>[4x]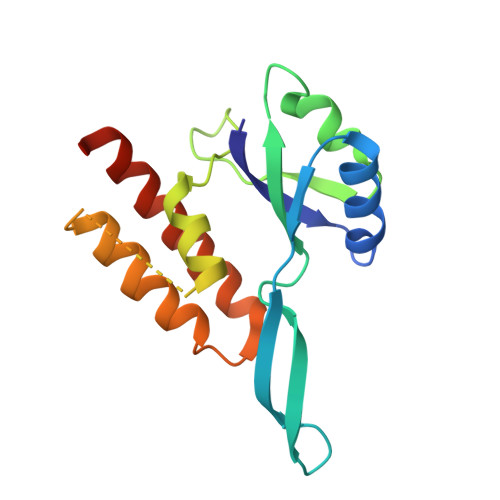MQSWYLLYCKRGQLQRAQEHLERQAVNCLAPMITLEKIVRGKRTAVSEPLFPNYLFVEFDPEVIHTTTINATRGVSHFVRFGASPAIVPSAVIHQLSVYKPKDIVDPATPYPGDKVIITEGAFEGFQAIFTEPDGEARSMLLLNLINKEIKHSVKNTEFRKL>GSDDSYARVRAVVMTRDDSSGGWLQLGGGGLSSVTVSKTLQPGDSGGTEFLVHGERLRDKTVILEC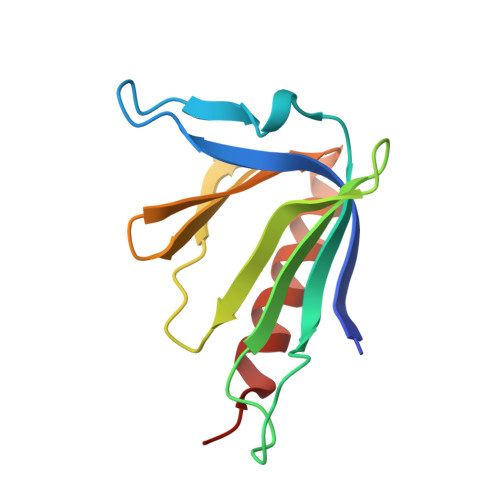VLRRDLVYNKVTPTFHHWRIGDKKFGLTFQSPADARAFDRGIRRAIEDLSQG[2x]> A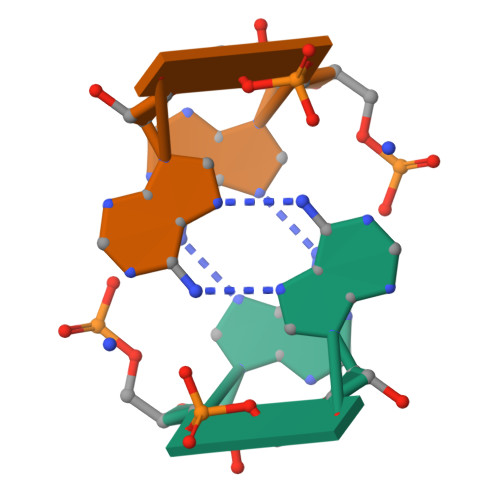AAAAAA2,2'-[(1R,1'R,3S,3'S)-6,6',9,9'-tetrahydroxy-1,1'-dimethyl-5,5',10,10'-tetraoxo-3,3',4,4',5,5',10,10'-octahydro-1H,1'H-8,8'-bibenzo[g]isochromene-3,3'-diyl]diacetic 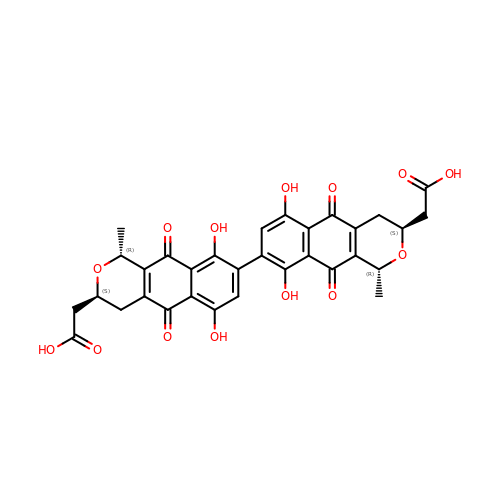acid | C32 H26 O14 | VTIKDEXOEJDMJP-WYUUTHIRSA-N> GPEFPNDYDFMEDILDETMKSTFKSEYPFEKRKAESERIADRFPNRIPVICEKAEKSDIPEIDKRKYLVPADLTVGQFVYVIRKRIMLPPEK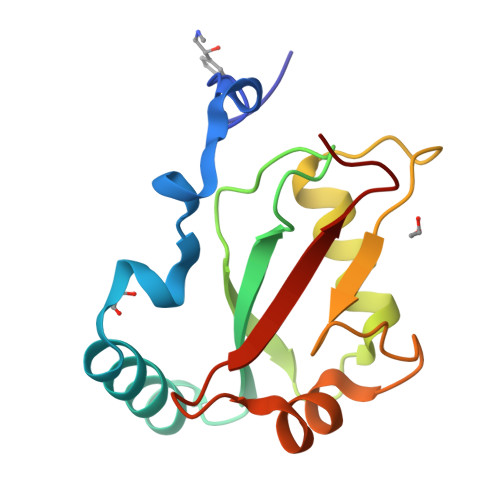AIFIFVNDTLPPTAALMSAIYQEHKDKDGFLYVTYSGENTFG PepT1 belongs to the solute carrier family 15 (SLC15), also known as the proton-coupled oligopeptide transporter (POT) family, which consists of four members in eukaryotes: PepT1 (SLC15A1), PepT2 (SLC15A2), PhT1 (SLC15A4), and PhT2 (SLC15A3). PepT1 and PepT2 are best characterized and mediate the uptake, distribution, and resorption of di- and tripeptides in the body. PepT1 and PepT2 are secondary active transporters, which are energized by the inward-directed electrochemical proton gradient. On a structural level, human PepT1 (HsPepT1) is 708 and human PepT2 (HsPepT2) is 729 amino acids long. Both polypeptides consist of a core transporter unit of predicted 12 transmembrane helices (TMs) of the major facilitator superfamily (MFS) fold and an extracellular immunoglobulin-like domain (ECD) placed between TM9 and TM10.

HsPepT1 was captured in the outward-facing conformation, both in apo and substrate-bound states, and in a substrate-bound outward-facing occluded structure. In this transition, salt bridges present on the intracellular side of all previous outward-facing states are disrupted, and a new one is established on the extracellular side, leading to the complete sealing from the luminal solvent. (C) Further bending of TM2 allows the interaction of H57, S302, N630, and D298 as a crucial step before (D) total sealing of the extracellular side and switching to the inward-facing occluded state stabilized by the salt bridge R185-D323.

> MGMSKSHSFFGYPLSIFFIVVNEFCERFSYYGMRAILILYFTNFISWDDNLSTAIYHTFVALCYLTPILGALIADSWLGKFKTIVSLSIVYTIGQAVTSVSSINDLTDHNHDGTPDSLPVHVVLSLIGLALIALGTGGIKPCVSAFGGDQFEEGQEKQRNRFFSIFYLAINAGSLLSTIITPMLRVQQCGIHSKQACYPLAFGVPAALMAVALIVFVLGSGMYKKFKPQGNIMGKVAKCIGFAIKNRFRHRSKAFPKREHWLDWAKEKYDERLISQIKMVTRVMFLYIPLPMFWALFDQQGSRWTLQATTMSGKIGALEIQPDQMQTVNAILIVIMVPIFDAVLYPLIAKCGFNFTSLKKMAVGMVLASMAFVVAAIVQVEIDKTLPVFPKGNEVQIKVLNIGNNTMNISLPGEMVTLGPMSQTNAFMTFDVNKLTRINISSPGSPVTAVTDDFKQGQRHTLLVWAPNHYQVVKDGLNQKPEKGENGIRFVNTFNELITITMSGKVYANISSYNASTYQFFPSGIKGFTISSTEIPPQCQPNFNTFYLEFGSAYTYIVQRKNDSCPEVKVFEDISANTVNMALQIPQYFLLTCGEVVFSVTGLEFSYSQAPSNMKSVLQAGWLLTVAVGNIIVLIVAGAGQFSKQWAEYILFAALLLVVCVIFAIMARFYTYINPAEIEAQFDEDEKKNRLEKSNPYFMSGANSQKQM;> AF>[2x]PSVYDAAAQLTADVKKDLRDSWKVIGSDKKGNGVALVTTLFADNQETIGYFKRLGDVSQGMANDKLRGHSITIMYAL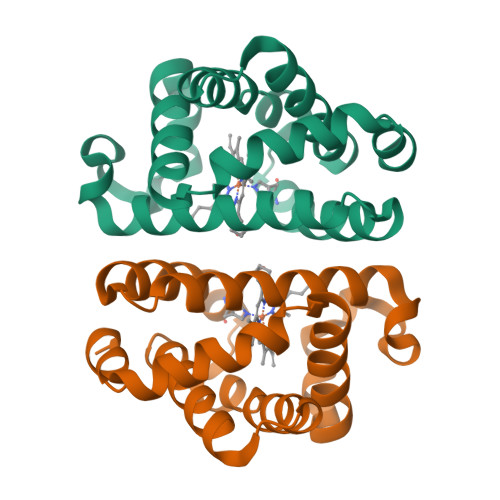QNFIDQLDNPDDLVCVVEKFAVNHITRKISAAEFGKINGPIKKVLASKNFGDKYANAWAKLVAVVQAAL> MASAAAEGEKGSPVVVGLLVVGNIIILLSGLALFAETIWVTADQYRVYPLMGVSGKDDVFAGAWIAIFCGFSFFVVASFGVGAALCRRRSMILTYLVLMLIVYIFECASCITSYTHRDYMVSNPSLITKQMLTFYSADSDQGRELTRLWDRVMIEQECCGTSGPMDWVNFTSAFRASTPEVVFPWPPLCCRRTGNFIPVNEEGCRLGHLDYLFTKGCFEHIGHAIDSYTWGISWFGFAILMWTLPVMLIAMYFYTTL;> MASPLPVRTLPLILILLAVLAPGASDFNISSLSGPLSPALTESLLVALPPCHLTGGNATLMVRRANDSKVVKSSFMVPPCRGRRELVSVVDSGSGFTVTRLSAYQVTNLVPGTKYYISYLVTKGASTESSREIPMSTLPRRKAEAIGLGMAPTGGMVVIQVLLSVAMFLLVVGFITALALGARK;> MPLLWALLALGCLQLGSGVNLQPQLASVTFATNNPTLTTVALEKPLCMFDSSAALHGTYEVYLYVLVDSASSRNASVQDSTKTPLSSTPQETEGGRTGPYKAAAFDLAPCSDLPSLDAVRDVSQASEILNAYLVRVGINGTCLSDPNFRGLCNPPLSAATEYRFKYVLVNISTGLVQDQTLWSDPVCTNQLTPYSAIDTWPGRRSGGMIVITSILGSLPFFLLVGFAGAIVLSLMDMGGADGEMTHDSQITQEAVPKGTSEPSYTSVNRGPPLDRAEVYASKLQD;> MAKDDSTVRCFQSLLVFGNVIIGMCGIALTAECIFFVSDQYSLYPLLEATDNDDIYGAAWIGIFVGICLFCLSVLGIVGIMKSNRKILLVYFILMFIVYGFEVASCITAATQRDFFTPNLFLKQMLERYQNNSPPSNDDKWKNNGVTKTWDRLMLQDYCCGVNGPSDWQKYTSAFRTENNDADYPWPRQCCVMNKLKEPLNLEACKLGVPGYYHNQGCYELISGPMNRHAWGVAWFGFAILCWTFWVLLGTMFYWSRIEY

The asymmetric unit membrane (AUM), primarily composed of the uroplakin complex, constitutes a critical permeability barrier in fulfilling this role. UPIa and UPIb have four transmembrane domains and belong to the tetraspanin family. Meanwhile, UPII and UPIIIa each possess a single transmembrane domain and form Ia/II and Ib/IIIa heterodimers within the endoplasmic reticulum (ER) in conjunction with UPIa and UPIb, respectively. The uroplakin complex also plays a crucial role in the development of urinary tract infections, as it facilitates Escherichia coli’s attachment to the urothelium.

In this study, we utilized cryo-electron microscopy to elucidate the three-dimensional structure of the uroplakin complex within the porcine AUM. Subsequently, we performed single particle analysis on AUM samples tilted up to 55°, resulting in a global resolution of 3.5 Å, with 3.2 Å and 6.3 Å resolutions in the transverse and vertical directions, respectively. Our findings unveiled that the uroplakin complexes are situated within hexagonally arranged crystalline lipid membrane domains, rich in hexosylceramides. However, our high-resolution reconstruction revealed that Ia/II and Ib/IIIa heterodimers constitute the outer and inner subdomains, respectively. However, our findings suggest that the prosequence forms the external surface of the complex through the formation of several beta sheets. Moreover, our reconstruction uncovered the presence of carbohydrate chains on six N-glycosylated residues, namely UPIa Asn169, UPIb Asn131, UPII Asn28, Asn57, UPIIIa Asn139, and Asn170 in accordance with previous studies. With these extracellular domains of UPII and UPIIIa, uroplakin heterotetramer overall adopts a Y-shaped conformation, which creates a substantial groove that may also provide a binding interface for other proteins (white arrow). Adjacent heterotetramers are connected through arches formed by the UPII and UPIIIa extracellular domains. Our map and model suggest that the hexameric complex is assembled through three inter-subunit interfaces: the Ia-Ib, II-IIIa, and IIIa-IIIa interfaces. The UPIIIa extends its loop 137–161 into the groove of an adjacent IIIa, forming an interface stabilized by a hydrophobic cluster composed of Pro146 of IIIa, Leu66, and Trp182 of the adjacent IIIa.>[2x]GSMTDGDYDYLIKLLALGDSGVGKTTFLYRYTDNKFNPKFITTVGIDFREKRVVYDTQGADGASGKAFKVHLQLWDTAGLERFRSLTTAFFR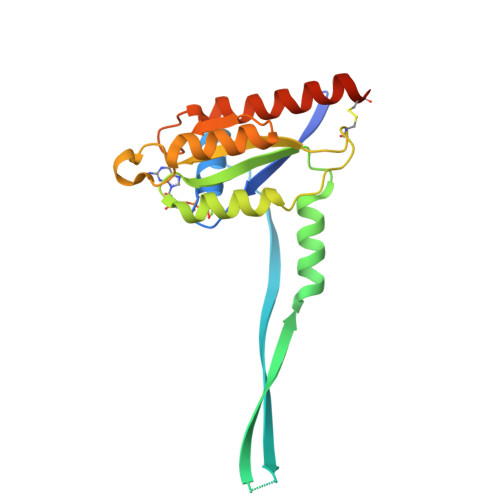DAMGFLLMFDLTSQQSFLNVRNWMSQLQANAYCENPDIVLIGNKADLPDQREVNERQARELAEKYGIPYFETSAATGQNVEKSVETLLDLIMKRMEKCVEKTQVPDTV> MAPTPQQVVQGTVDELLSDIKANKAAYKADPQKLYATLDRILGPVVDAEGIAKSVMTVKYSRQASPEQIKRFEEVFKNSLMQFYGNALLEYDNQDIRVLPSSAKPSDDRASVNMEI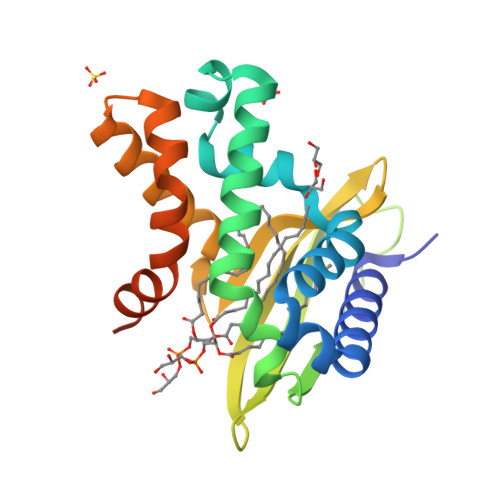RDSKGTVYPVSYTMTNLAGGWKVRNVIINGINIGKLFRDQFADTMQKNRNDLEKTIAGWGEVVAKAKETAKAEEAGAKKLAAALEHHHHHH>MKERILQEIKTRVNRKSWELWFSSFDVKSIEGNKVVFSVGNLFIKEWLEKKYYSVLSKAVKVVLGNDATFEITYEAFEPHSSYSEPLVKKRAVLLTPLNPDYTFENFVVGPGNSFAYHAALEVAKHPGRYNPLFIYGGVGLGKTHLLQSIGNYVVQNEPDLRVMYITSEKFLNDLVDSMKEGKLNEFREKYRKKVDILLIDDVQFLIGKTGVQTELFHTFNELHDSGKQIVICSDREPQKLSEFQDRLVSRFQMGLVAKLEPPDEETRKSIARKMLEIEHGELPEEVLNFVAENVDDNLRRLRGAIIKLLVYKETTGKEVDLKEAILLLKDFIKPNRVKAMDPIDELIEIVAKVTGVPREEILSNSRNVKALTARRIGMY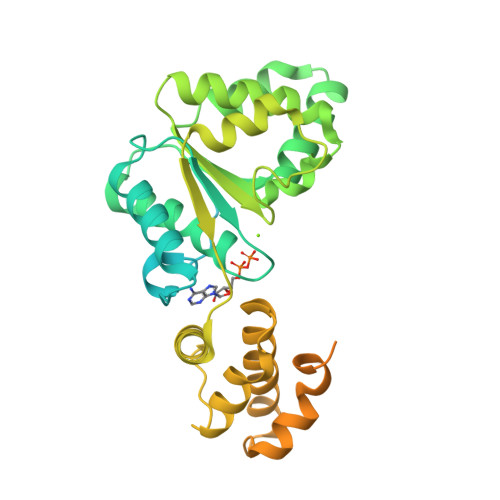VAKNYLKSSLRTIAEKFNRSHPVVVDSVKKVKDSLLKGNKQLKALIDEVIGEISRRALSG[3x]~{N}-[(2~{S},3~{R},4~{R},5~{R},6~{R})-2-[(2~{R},3~{S},4~{R},5~{R},6~{S})-5-acetamido-2-(hydroxymethyl)-6-(4-nitrophenoxy)-4-oxidanyl-oxan-3-yl]oxy-6-(hydroxymethyl)-4,5-bis(oxidanyl)oxan-3-yl]ethanamide 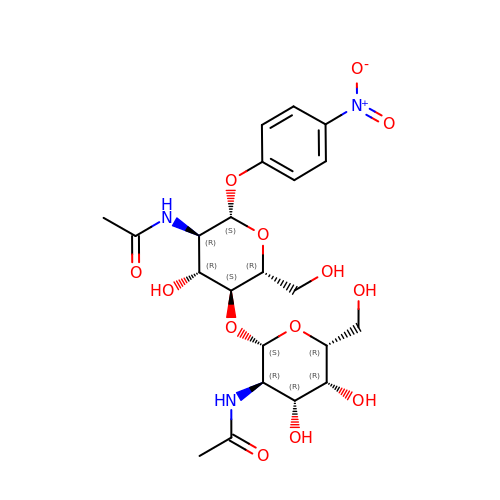| C22 H31 N3 O13 | HWBFEVWOQMUQIE-BFKOZBEUSA-N> AMPVFHTRTIESILEPVAQQISHLVIMHEEGEVDGKAIPDLTAPVSAVQAAVSNLVRVGKETVQTTEDQILKRDMPPAFIKVENACTKLVRAAQMLQADPYSVPARDYLIDGSRGILSGTSDLLLTFDEAEVRKIIRVCKGILEYLTVAE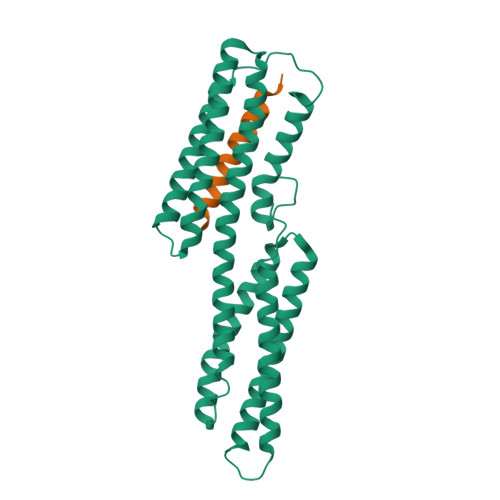VVETMEDLVTYTKNLGPGMTKMAKMIDERQQELTHQEHRVMLVNSMNTVKELLPVLISAMKIFVTTKNTKSQGIEEALKNRNFTVEKMSAEINEIIRVLQLTSWD;> GRPLLQAAKGLAGAVSELLRSAQP>[2x]MNLVLMGLPGAGKGTQGERI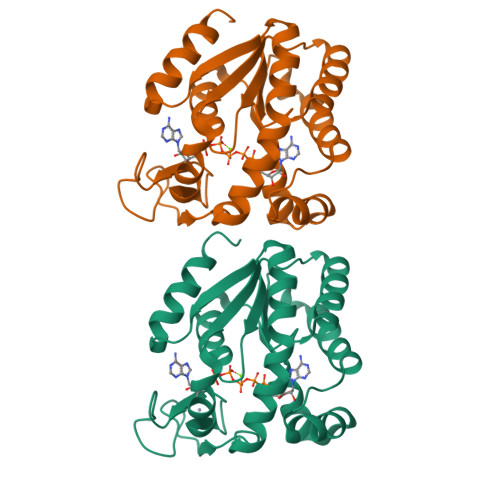VEDYGIPHISTGDMFRAAMKEETPLGLEAKSYIDKGELVPDEVTIGIVKERLGKDDCERGFLLDGFPRTVAQAEALEEILEEYGKPIDYVINIEVDKDVLMERLTGRRICSVCGTTYHLVFNPPKTPGICDKDGGELYQRADDNEETVSKRLEVNMKQTQPLLDFYSEKGYLVNVNGQRDIQDVYADVKDLLGGLK>[3x]GSP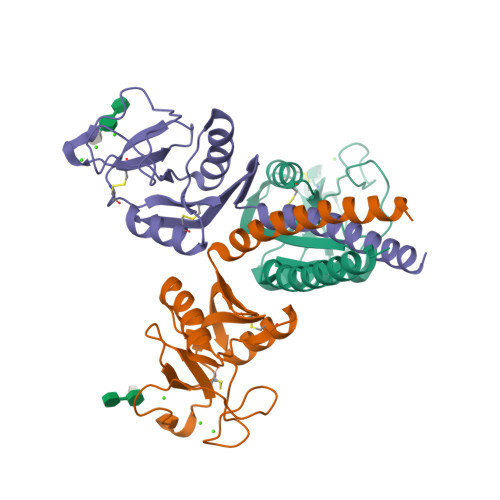GLKGDKGIPGDKGAKGESGLPDVASLRQQVEALQGQVQHLQAAFSQYKKVELFPNGQSVGEKIFKTAGFVKPFTEAQLLCTQAGGQLASPRSAAENAALQQLVVAKNEAAFLSMTDSKTEGKFTYPTGESLVYSNWAPGEPNDDGGSEDCVEIFTNGKWNDRACGEKRLVVCEF In this study, we focus on KKT14 and KKT15, proteins of unknown functions that localize at the kinetochore from G2 until the end of anaphase in T. brucei. Here, we discover that KKT14 has a pseudokinase domain in its C-terminus, which is most similar to the kinase domain of Bub1. The N-terminal part of KKT14 interacts with KKT15, which we suggest to be a Bub3 orthologue. In this study, we propose that the kinetoplastid kinetochore proteins KKT14 and KKT15 are divergent Bub1/BubR1 and Bub3 orthologues, respectively.

By screening four kinetoplastid species (T. brucei, T. cruzi, Paratrypanosoma confusum and Apiculatamorpha spiralis), we succeeded in determining a 2.2 Å resolution crystal structure for the C-terminal domain of the KKT14 protein from the prokinetoplastid A. spiralis (clone PhF-6). Apiculatamorpha spiralis KKT14365−640 crystallized with two molecules in an asymmetric unit. Both molecules were essentially identical except for minor variations in flexible loops. Interestingly, a structural homology search using the distance-matrix alignment (DALI) server revealed similarity to a protein kinase fold with an N-lobe and C-lobe. The N-lobe contains a five-stranded β-sheet, a helix termed the C-helix (αC), and loops that correspond to the catalytic loop and activation loop, while the C-lobe comprises a bundle of α-helices. Although most protein kinases share a similar fold, we found that the most similar structure of A. spiralis KKT14365−640 in the PDB database was the Bub1 kinase domain. Human Bub1 was the top hit in the DALI search with a Z-score of 15.5, while the next best hit was the MST3 kinase (Z-score 13.0). The higher structural similarity of KKT14 to the kinase domain of Bub1 rather than other kinases is owing to an N-terminal extension that is present in Bub1 and KKT14. In the crystal structure of A. spiralis KKT14, W548 (the phenylalanine equivalent of the DFG motif, which is CWD in A. spiralis KKT14), strictly conserved among kinetoplastids, faces away from the active site. Similarly, in both the crystal structure of A. spiralis KKT14 and the AlphaFold2-predicted structure of T. brucei KKT14, the N-terminal extension makes extensive contacts with the N-lobe, which may stabilize the pseudokinase structure.

>GSELAHFQSEIEENYEAVGNVVVDLMGGCEPTLRVGRVQLGNDIFTLREEIRATELKRVLYVGTTEGDEFPVVVYAWTNGNSYESAKAFVASQGLNVPCRIVGYRSYDKMSGYTAIIFPQGHVYSLRTFLQRSVPTRATETALYYVAETLRSLCTRRIIHCALTPDNVFMYMDSTGASLKTFPVCWDDCVDAAMFSERGLKFVPSLPVLMRHAVKEIDGSYIDFVSFCRMFRQIENNCSAMCQKVAKMKAPPVVRMTDYTNIQTELTWDMDAVMNHFC[2x]>[4x]AMGQRAMKFCQGVVRELMSKKYASFNYPFLEPVDPVALNCPTYFDYVKEPMDLGTVSKKLSNWEYENLDQAEHDIRLIFQNCYAFNPDGTIVNMMGHRLEDIFNTKWADRPLYSDVES

The fungal Bromodomain and Extra‐Terminal (BET) protein Bdf1 is a potential antifungal target against invasive fungal infections. One attractive target is the fungal BET protein Bdf1, a global transcriptional regulator. BET proteins bind chromatin through their two bromodomains (BDs), BD1 and BD2, which specifically recognize histones acetylated on lysines. We show that Bdf1 is essential in C. glabrata, and that inactivation of both Bdf1 BDs induces lethality.

We next assessed the ability of small molecules to differentially inhibit human BET and CgBdf1 BDs by evaluating the ability of BETi compounds JQ1, I‐BET151, bromosporine (BSP) and PFI‐1 to inhibit binding to an H4ac4 peptide in a homogeneous time‐resolved fluorescence (HTRF) assay. While these compounds potently inhibited human Brd4 BD1 and BD2 (IC50 values of ≈10–100 nM), consistent with previous reports, they inhibited CgBdf1 BDs more weakly (IC50 values between 0.5 and >100 µM; i.e., a 10‐ to 1000‐fold reduction in sensitivity) and failed to inhibit C. glabrata growth in vitro. These results demonstrate that small molecules can strongly discriminate between human BET and CgBdf1 BDs. To rationalize these data, we determined the crystal structure of the highest affinity CgBD/BETi complex, CgBD2 bound to I‐BET151. CgBD2 undergoes a minor conformational change to accommodate IBET‐151: in unbound CgBD2, the side chain of “YPF‐shelf” residue Tyr327 adopts a gauche minus (g−) conformation, stabilized by a sulfur‐π interaction with residue Met395, whereas, in the complex, Tyr327 adopts the trans conformation to avoid a steric clash with I‐BET151, thereby widening the ligand binding pocket. The shorter side chains (Cys340, Val392) and altered conformation (Glu331) of three CgBD2 residues further widen the binding pocket and reduce the number of hydrophobic contacts with I‐BET151. Consistent with this observation, the Brd4 BD1 pocket buries more of the ligand's solvent‐accessible surface area (SASA) compared to CgBD2 (55.4% vs. 47.2%). The looser fit of these BETi compounds within the more spacious CgBD1 and CgBD2 binding pockets explains their reduced potency relative to human BET BDs.>MRQVDAATHGGRAVIELREKILSGELPGGMRLFEVSTAELLDISRTPVREALSRLTEEGLLNRLPGGGFVVRRFGFADVVDAIEVRGVMEGTAARLAAERGVSKVALEEIDATVQQLDLCFGDRVDDVDFDGYAALNRIFHHQLAALCGSEMIRREVERASSLPFASPSAFLPDKANIGAFRRSLRGAQEQHKAIVAAIVAREGARAEAVAREHSRTARTNLEYMIREAPELIAQVPGLALISDHHHHHH[2x]

Here, we characterized Atu1419 as a transcriptional repressor of its own repression in addition to two other genes (atu1418 and atu1420). The structures revealed Atu1419 to be a member of the VanR group of the FadR C-terminal domain (FCD; Pfam PF07729) subfamily of the large GntR superfamily of transcriptional factors (>93 135 members in Pfam database). Like FadR, Atu1419 possesses a characteristic molecular architecture, composed of a conserved N-terminal DNA binding domain containing the wHTH motif and a C-terminal effector binding/oligomerization domain. We identified the short palindromic region composed of 10 base pairs and a degenerated palindrome bound to Atu1419 and the N5,N10-methylenetetrahydrofolate (MEF) as the effector molecule disrupting Atu1419-DNA interaction, allowing the expression of the second part of the HCA degradation pathway.

The orientation B of the citrate was also observed in another structure of Atu1419 solved at a higher resolution of 1.75 Å but in a different space group (P21212). Here, two similar monomers (RMSD of 0.98 Å for all Cα atoms) are in the asymmetric unit and form a dimer, which in turn form a tetramer by the crystal symmetry with globally unchanged dimer interfaces (1553 and 701 Å2 per subunit for dimers AB and AD, respectively) compared with those from the P212121 structure. They resemble subunits B/C/D of the P212121 structure and bind similarly a citrate molecule. Nonetheless, their citrates are slightly shifted by 0.6 Å toward Arg86 losing the interaction with Asn221 compared with those in the P212121 structure.ethyl (3R)-4-cyano-3-hydroxybutanoate | C7 H11 N O3 | 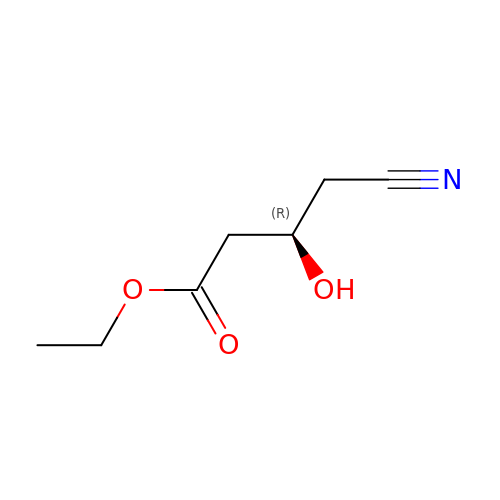LOQFROBMBSKWQY-ZCFIWIBFSA-N(7R)-N-benzyl-1,7-diethyl-2,3,6,7-tetrahydro-1H-1,4-diazepine-7-carboxamide 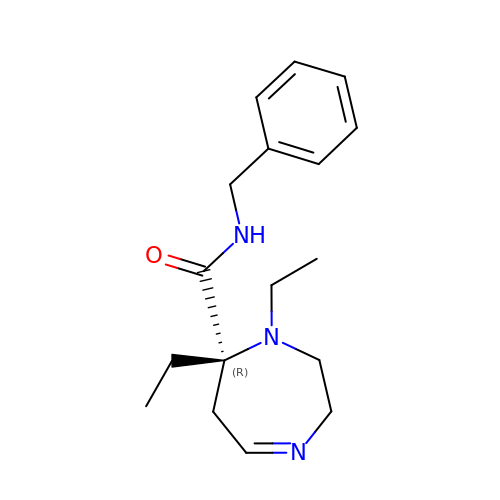| C17 H25 N3 O | ZQBDTUTZFRWAGO-QGZVFWFLSA-N> MSLPAHLQQTFSPEEIQFIVENEPIKIFPRITTRQKIRGDDRGTGNHTRWQLITTDDKALNNMVAMRSTEVVL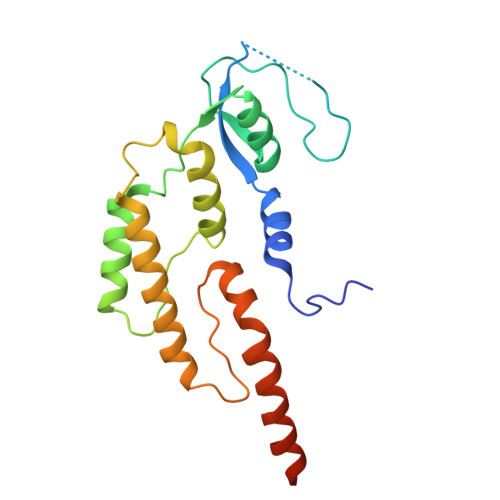WIALLLKQQSKCSIVAPQWLTTKELDRKIQYEKTHPDRFSELPWNWLVLARILFNKAKDDFHDPIHELRGKIQDLREIRQIKVLKGLKYLNESHLQLDNLSLLEINELRPFITEIMDKLREIHTASLTAGTENDEEEFNI>[2x]ASKWTYFGPDGENSWSKKYPSCGGLLQSPIDLHSDILQYDASLTPLEFQGYNLSANKQFLLTNNGHSVKLNLPSDMHIQGLQSRYSATQLHLHWGNPNDPHGSEHTVSGQHFAAELHIVHYNSDLYPDASTASNKSEGLAVLAVLIEMGSFNPSYDKIFSHLQHVKYKGQEAFVPGF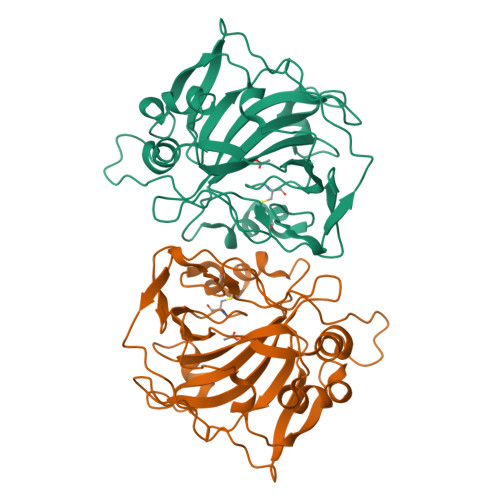NIEELLPERTAEYYRYRGSLTTPPCNPTVLWTVFRNPVQISQEQLLALETALYCTHMDDPSPREMINNFRQVQKFDERLVYTSFSQ> MWLFFFALAVIYMIYKRDVFKKIAVNLKMNGVSIPFVDKYSKQYPTYTKNALFHVTRFNN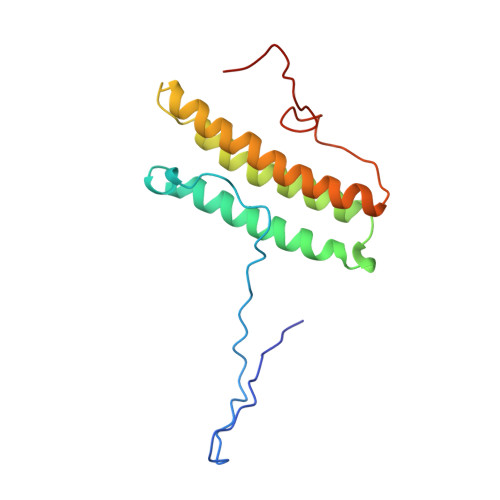AYQKTFEYKNISIDTINNLFSIRDDVLYNISEIKLRLPNDLTQEKEINYMYEKTDQRLMEYITDVKSRFHINIYPGTMSSAFEARNYRASNDIVF> GHGNNKEPNTKNRLDSAEKKKKMSVQAEIGILDHVDGSSEFVSQDTKVICSV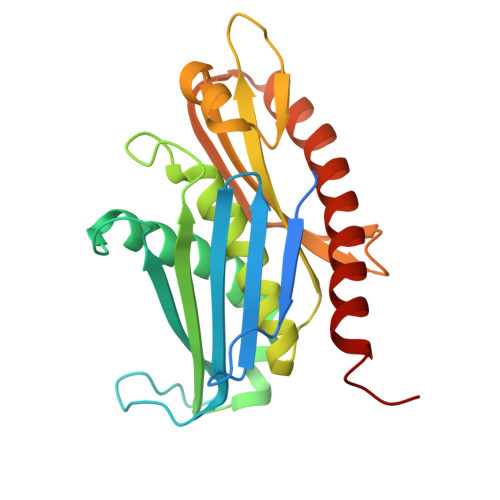TGPIEPKARQELPTQLALEIIVRPAKGVATTREKVLEDKLRAVLTPLITRHCYPRQLCQITCQILESGEDEAEFSLRELSCCINAAFLALVDAGIALNSMCASIPIAIIKDTSDIIVDPTAEQLKISLSVHTLALEFVNGGKVVKNVLLLDSNGDFNEDQLFSLLELGEQKCQELVTNIRRIIQDNISPRLVV>EPTCNTPSNRACWSDGFDINTDYEVSTPDTGVTQSYVFNLTEVDNWMGPDGVVKEKVMLINGNIMGPNIVANWGDTVEVTVINNLVTNGTSIHWHGIHQKDTNLHDGANGVTECPIPPKGGQRTYRWRARQYGTSWYHSHFSAQYGNGVVGTIQINGPASLPYDIDLGVFPITDYYYRAADDLVHFTQNNAPPFSDNVLINGTAVNPNTGEGQYANVTLTPGKRHRLRILNTSTENHFQVSLVNHTMTVIAADMVPVNAMTVDSLFLAVGQRYDVVIDASRAPDNYWFNVTFGGQAACGGSLNPHPAAIFHYAGAPGGLPTDEGTPPVDHQCLDTLDVRPVVPRSVPVNSFVKRPDNTLPVALDLTGTPLFVWKVNGSDINVDWGKPIIDYILTGNTSYPVSDNIVQVDAVDQWTYWLIENDPEGPFSLPHPMHLHGHDFLVLGRSPDVPAASQQRF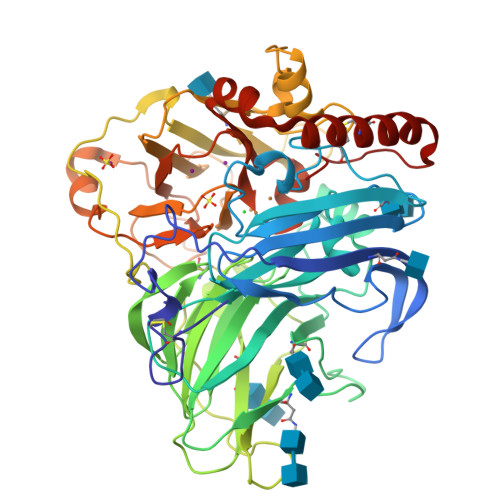VFDPAVDLARLNGDNPPRRDTTMLPAGGWLLLAFRTDNPGAWLFHCHIAWHVSGGLSVDFLERPADLRQRISQEDEDDFNRVCDEWRAYWPTNPYPKIDSGL[2x]> MSAEKLFTPLKVGAVTAPNRVFMAPLTRLRSIEPGDIPTPLMGEYYRQRASAGLIISEATQISAQAKGYAGAPGLHSPEQIAAWKKITAGVHAEDGRIAVQLWHTGRASHSSIQPGGQAPVSASALNANTRTSLRDENGNAIRVDTTTPRALELDEIPGIVNDFRQAVANAREAGFDLVELHSAHGYLLHQFLSPSSNQRTDQYGGSVENRARLVLEVVDAVCNEWSADRI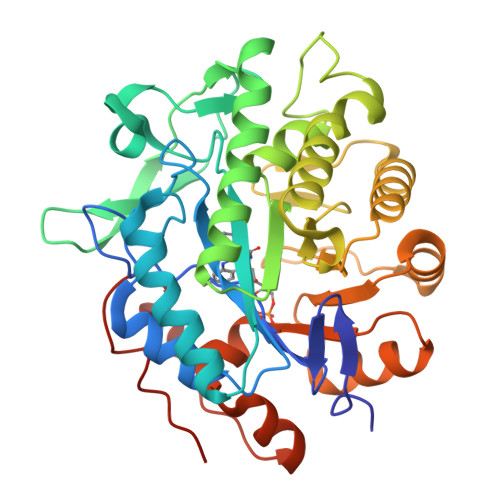GIRVSPIGTFQNVDNGPNEEADALYLIEELAKRGIAYLHMSETDLAGGKPYSEAFRQKVRERFHGVIIGAGAYTAEKAEDLIGKGLIDAVAFGRDYIANPDLVARLQKKAELNPQRPESFYGGGAEGYTDYPSLHHHHHHHH> MSQGTLYANFRIRTWVPRGLVKALKLDVKVVTPDAAAEQFARDFPLKKVPAFVGPKGYKLTEAMAINYYLVKLSQDDKMKTQLLGADDDLNAQAQIIRWQSL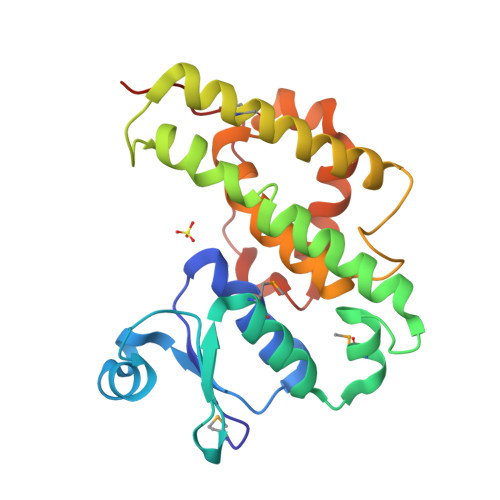ANSDLCIQIANTIVPLKGGAPYNKKSVDSAMDAVDKIVDIFENRLKNYTYLATENISLADLVAASIFTRYFESLFGTEWRAQHPAIVRWFNTVRASPFLKDEYKDFKFADKPLSPPQ>GSSSLIRRVISTAKAPGAIGPYSQAVLVDRTIYISGQIGMDPSSGQLVSGGVAEEAKQALKNMGEILKAAGCDFTNVVK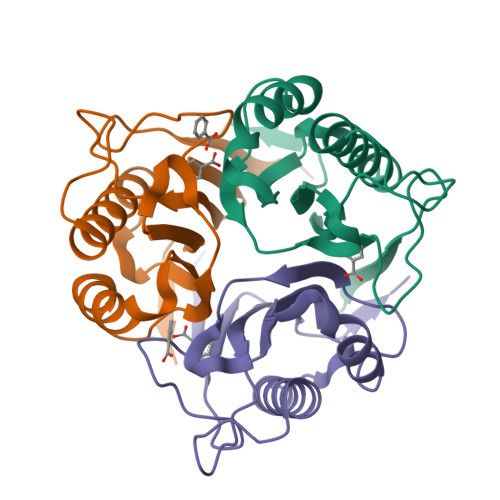TTVLLADINDFNTVNEIYKQYFKSNFPARAAYQVAALPKGSRIEIEAVAIQGPLTTASL[9x]>SNGLMAKRLRRELLNTYEQLGKSGLPFLDDIGKVDVKFGLSLQLLKSIEQRGMGFNSIGTFKAIVKLSWVDTILRWDPEPPFDFQKIEISPDEIWTPDIKLFNSVDLDMTLDRTTQAIVFSNGTVLWIPPAVLKVL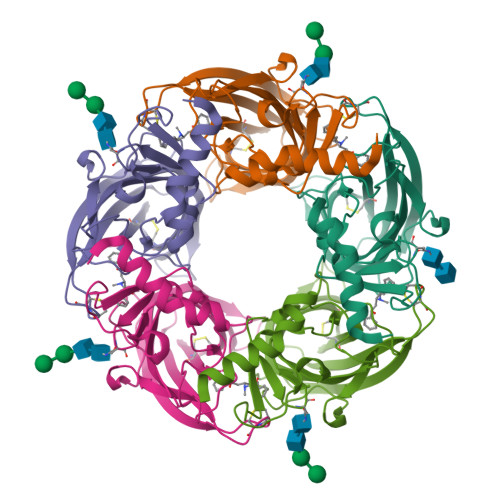CVSQDDVDSCHFQFGSWVYSVDEVDIHFMDDKAEVLLDFYQDSLEILENSAQRQEVVYPCCESAYVEMKYLLALRSENGNSTYSRDLAHHHHHH[5x]> RPPKP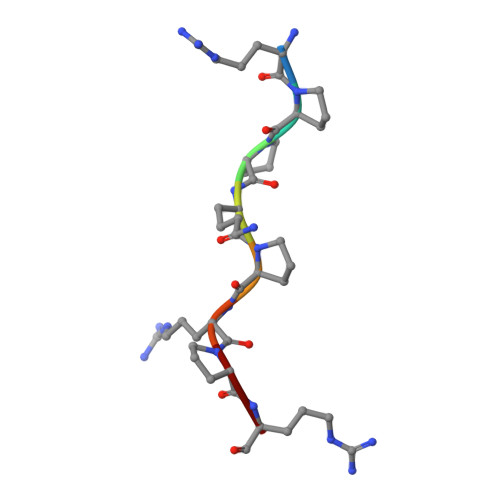RPR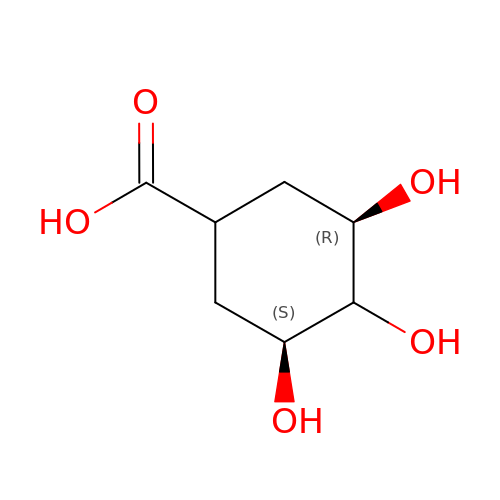(3~{R})-3,4,5-tris(hydroxyl)cyclohexane-1-carboxylic acid | C7 H12 O5 | SOWVWGZSLABJMC-HMWJNGDSSA-N The homodimeric 6-phosphofructo-2-kinase/fructose-2,6-bisphosphatases (PFKFBs) are key regulatory enzymes in the glycolysis. These bifunctional enzymes synthesize and degrade fructose-2,6-bisphosphate (F-2,6-P2), which acts as an allosteric activator for the rate-limiting enzyme and committed step in glycolysis, i.e., 6-phophofructo-1-kinase (PFK-1). In contrast to the PFKFB isoforms 1, 2, and 4, which are constitutively expressed in testes/kidney/heart and liver/muscle, PFKFB3 is an inducible isoform9 with increased expression in response to hypoxia, extracellular acidosis, and inflammation. PFKFB3 also stands out with a kinase to bisphosphatase ratio of 740:1, while the other isoforms display a more balanced ratio closer to unity.

Competition experiments with ATP were used to identify ATP-competitive and non-ATP-competitive binders. This effort lead to the identification and further development of a series of phenylsulfonamido salicylic acids that rendered sub-µM inhibitors of PFKFB3. Significant cross-reactivity is only observed for PFKFB4, although the selectivity window is about 20-fold with IC50 values of 0.19 and 3.6 µM, respectively. The sub-µM potency for PFKFB3 was also confirmed using isothermal titration calorimetry as illustrated in Figure S6D and co-crystal structures demonstrated binding in the active site, mimicking several of the interactions made by the endogenous substrate fructose-6-phosphate (F6P). Further characterization of KAN0438241 and its ester KAN0438757, which was designed to increase cell permeability and efficient intracellular hydrolysis to release the active compound, involved examination of their impact on the proximal biomarker F-2,6-P2 in several different cell lines. The effect on intracellular F-2,6-P2 levels is in contrast to what we observed in the in vitro enzymatic assay for PFKFB3, where the ester is largely inactive. Given the binding pose, which involves important interactions for the carboxylate, the lack of activity for the ester in a non-cellular setting is not surprising. To further validate KAN0438241 as a useful chemical tool for probing cellular PFKFB3 activity, we examined the kinome-wide selectivity profile of KAN0438757 and its active metabolite KAN0438241 with DiscoveRx’s KINOMEscan technology. Both compounds displayed high selectivity (SScore(35) = 0) at 2 µM.

> MPLELTQSRVQKIWVPVDHRPSLPRSCGPKLTNSPTVIVMVGLPARGKTYISKKLTRYLNWIGVPTKVFNVGEYRREAVKQYSSYNFFRPDNEEAMKVRKQCALAALRDVKSYLAKEGGQIAVFDATNTTRERRHMILHFAKENDFKAFFIESVCDDPTVVASNIMEVKISSPDYKDCNSAEAMDDFMKRISCYEASYQPLDPDKCDRDLSLIKVIDVGRRFLVNRVQDHIQSRIVYYLMNIHVQPRTIYLCRHGENEHNLQGRIGGDSGLSSRGKKFASALSKFVEEQNLKDLRVWTSQLKSTIQTAEALRLPYEQWKALNEIDAGVCEELTYEEIRDTYPEEYALREQDKYYYRYPTGESYQDLVQRLEPVIMELERQENVLVICHQAVLRCLLAYFLDKSAEEMPYLKCPLHTVLKLTPVAYGCRVESIYLNVESVCTHRERSEDAKKGPNPLMRRNSVTPLASPEPTKKPRINSFEEHVASTSAALPSCLPPEVPTQLPGQNMKGSRSSADSSRKH> ARARKGALVQCDPSIKALI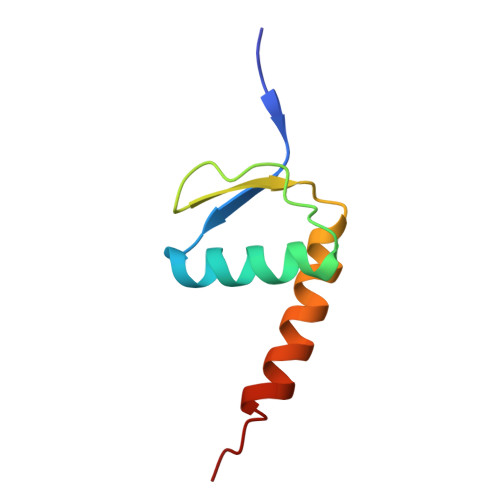LQIDAKMSDIVLEELDDTHLLVNPSKVEFVKHELNRLLSKNIYNPMD> GPMPFYDSRPPEGWPKGSINDMDYPLLGSICAVCCVFVAGSGIWMLYRLDLGMGYSCKPYKSGRAPEVNSLSGIICLLCGTMYAAKSFDFFDGGGTPFSLNWYWYLDYVFTCPLLILDFAFTLDLPHKIRYFFAVFLTLWCGVAAFVTPSAYRFAYYALGCCWFTPFALSLMRHVKERYLVYPPKCQRWLFWACVIFFGFWPMFPILFIFSWLGTGHISQQAFYIIFAFLDLTCKSIFGILMTVFRLELEEHTEVQGLPLNEPETLSLEVLFQ

KCR channelrhodopsins (K+-selective light-gated ion channels) have received attention as potential inhibitory optogenetic tools but more broadly pose a fundamental mystery regarding how their K+ selectivity is achieved. Here, we present 2.5–2.7 Å cryo-electron microscopy structures of HcKCR1 and HcKCR2 and of a structure-guided mutant with enhanced K+ selectivity. Structural, electrophysiological, computational, spectroscopic, and biochemical analyses reveal a distinctive mechanism for K+ selectivity; rather than forming the symmetrical filter of canonical K+ channels achieving both selectivity and dehydration, instead, three extracellular-vestibule residues within each monomer form a flexible asymmetric selectivity gate, while a distinct dehydration pathway extends intracellularly.

In contrast, the reason behind the significant enhancement of K+ selectivity we observed in H225 mutations remained unclear, as H225 is not directly involved in the selectivity triad. To address this, we determined the cryo-EM structure of the H225F mutant at 2.7 Å resolution and compared it to WT, initially observing no remarkable differences in the EV. While H225 is not part of the selectivity triad, it interacts weakly with W102 and Y222 due to its proximity. Considering that mutations in H225 might affect stability of the selectivity filter, we conducted additional MD simulations for both WT and H225F. Surprisingly, in simulations of the H225F mutant, Y222 occupies the tight conformation for a greater fraction than in WT simulations; simulations of the H225A mutant (also with greater K+ selectivity) using our homology model revealed the same trend. These results strongly suggest that the selectivity triad in HcKCR1 has intrinsic flexibility and that mutation to H225 stabilizes the architecture favoring K+ selectivity. However, a pronounced discrepancy was observed in K+ vs. Li+ permeability between WT and H225F (Erev for WT = −102.8 ± 2.7 mV vs. Erev for H225F = −119.2 ± 2.3 mV; p = 0.0035). These findings further support the idea that the selectivity conferred by the triad and its enhancement by H225F depend upon the hydration radius of cations entering from the extracellular side. The H225F mutant exhibited hyperpolarized Erev compared to WT (-69.6 ± 1.9 mV vs. -82.0 ± 1.9 mV; p = 0.0004) with only slightly decreased photocurrents and comparable kinetics in cultured neurons. Because of these potent loss-of-function properties, we name the H225F mutants of HcKCR1 and 2 as KALI-1 and KALI-2 (K+-selectivity Augmented Light-Gated Ion Channels).>[2x]MAPFEIPDRYKKPAKMLHEICIAESGASEEQLRTCLDGTVPTAPAAKCYIHCLFDKIDVVDEATGRILLDRLLYIIPDDVKAAVDHLTRECSHIVTPD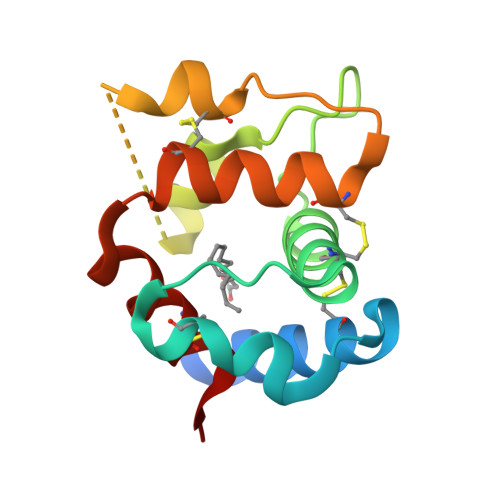KCETAYETVKCYFNAHDEVIKFCHLLVLE>GAMSDPDLEATLRAIVHSATSLVDARYGAMEVHDRQHRVLHFVYEGIDEETVRRIGHLPKGLGVIGLLIEDPKPLRLDDVSAHPASIGFPPYHPPMRTFLGVPVRVRDESFGTLYL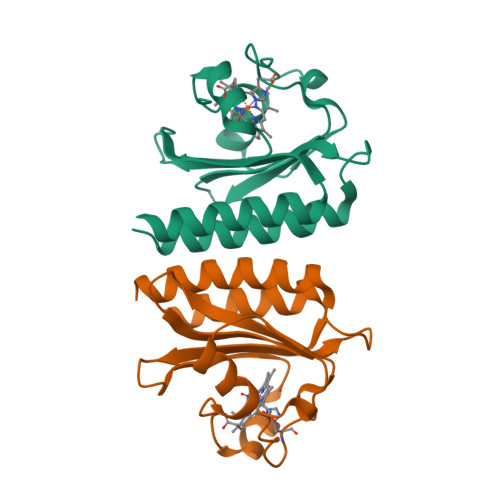TDKTNGQPFSDDDEVLVQALAAAAGIAVANARLYQQAK[2x]> MDEYVQELKGLIRKHIPERCEFGHQKVTFLSQVHPSPLLTEGFKLLSSLVELESCEAHACQANTDQRFVDVILSDNGILCPTLPKVIPDGFKLTGKTLILLETFVRVNPDEFEKKWKADMSKLLNLKHDLQKSGVTLVPIVDGRSNYNNRFVADWVIERIRWLLIEILKASKSMLEIDIEDQEYQRLIHSLSNVKNQSLGLENLEHLKRNSLDYDERLNESLFIGLKGDIRESTVREELIKLKLWFKDEVFSKGLGKFKLTDRRELLESLSSLGAHLDSDVSSCPFCNNKLMEIVYNVTFSCVERTDGVATVDQQFSTTHSNIEKHYLSVLSLCNKIKGLKVFNTRRNTLLFLDLIMVNLMVDISDSCQDAIESLRKSGLIVGQMVMLVNDRVLDILEAVKLIRKKIGTNPNWVKNCSKILERSHPEIWHHLSTLIKQPDFNSLISIAQHLVSDRPIMRYSVERGSDKICRHKLFQEMSSFEQMRLFKTLSSISLSLINSMKTSFSSRLLVNEREFSKYFGNVRLRECYAQRFYLAESLVGFLFYQKTGERSRCYSVYLSDNGVMSEQGSFYCDPKRFFLPVFSDEVLAGMCEEMTSWLDFDTGLMNDTGPILRLLVLAILCSPSKRNQTFLQGLRYFLMAFANQIHHIDLTSKLVVECKSSSEVVVQRLAVGLFIRLLSGESDASLFFSRRFKYLLNVSYLCHLITKETPDRLTDQIKCFEKFIEPKVKFGCAVVNPSLNGKLTVDQEDIMINGLKKFFSKSLRDTEDVQTPGVCKELLNYCVSLFNRGKLKVSGELKNNPFRPNITSTALDLSSNKSVVIPKLDELGNILSTYDKEKLVSACVSSMAERFKTKGRYNLDPDSTDYLILKNLTGLVSAGPKAKSTQEELSLMYEALTEEQVESFNEIKHDVQVALAKMADNSVNTRTKNLGRADNSVKNGNNPLDNLWSPFGVMKEIRAEVSLHEVKDFDPDVLPPEVYKELCDAVYKSSEKCNFFLEGVLDVCPLGLLLKNLTTSSYVDEEYFMCFKYLLI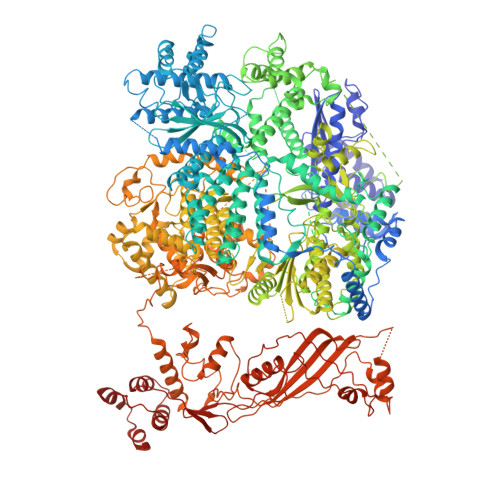QGHFDQKLGSYEHKSRSRLGFTDETLRLKDEVRLSIRESNSEAIADKLDKSYFTNAALRNLCFYSEDSPTEFTSISSNSGNLKFGLSYKEQVGSNRELYVGDLNTKLMTRLVEDFSEAVGNSMKYTCLNSEKEFERAICDMKMAVNNGDLSCSYDHSKWGPTMSPALFLALLQMLELRTPVDRSKIDLDSVKSILKWHLHKVVEVPINVAEAYCIGKLKRSLGLMGCGSTSLSEEFFHQTMQLNGQIPSHIMSVLDMGQGILHNTSDLYGLITEQFLCYALDLLYDVIPVSYTSSDDQITLIKTPSLDIEGGSDAAEWLEMICFHEFLSSKLNKFVSPKSVIGTFVAEFKSRFFVMGEETPLLTKFVAAALHNVKCKTPTQLSETIDTICDQCIANGVSTKIVTRISKRVNQLIRYSGYGETPFGAIEDQDVKDWVDGSRGYRLQRKIEAIFHDDKETSFIRNCARKVFNDIKRGRIFEENLINLIGRGGDEALTGFLQYAGCSEQEVNRVLNYRWVNLSSFGDLRLVLRTKLMTSRRVLEREEVPTLIKTLQSKLSRNFTKGVKKILAESINKSAFQSSVASGFIGFCKSMGSKCVRDGKGGFLYIKEVYSGVSACTCEICALKPKIIYCNNSLNKVSQFSKPILWDYFSLVLTNACELGEWVFSTVKEPQKPLVLNNQNFFWAVKPKVVRQIEDQLGMNHVLQSIRRNYPVLFDEHLTPFMNDLQVSRTMDSGRLKFLDVCIALDMMNENLGIISHLLKTRDNSVYIVKQSDCALAHIRQSSYTDWELGLSPQQICTNFKTQLVLSSMVNPLVLSTSCLKSFFWFNEVLELEDDSQIELAELTDFALMVKNQNVSRAMFVEDIAMGYVVSNFEGVRISLSNVMVDGVQLPPQEKAPDIGELFGLKAENVIVGLVVQIDHVRMSTKFKLKRKMVYSFSLECIMDVGEIQNKEVILKVVAVDQSVSGSGGNHMLLDGVSVVASLPLFTGQASFDLAAMLIESNLAGSNDNFLMRNVTLDLGGFSPELSDKYSYRLSGPENQEDPLVLKDGAFYVGGERLSTYKVEFTGDLVVKALGALEDDESVVSMLHQLWPYLKATSQVILFQQEDFTIVHDLYKKQLTKSIESFGEWIEFTNFKVAYSKSLKELVISDTQGSFRLKGVMCRPLASTPQVEDIE>GPGSPITDERVYESIGQYGGETVKIVRIEKARDIPLGATVRNEMDSVIISRIVKGGAAEKSGLLHEGDEVLEINGIEIRGKDVNEVFDLLSDMHGTLTFVLIPSQQIKPPPAKETVIHVKAHFDYDPSDDPYVPCRELGLSFQKGDILHVISQEDPNWWQAYREGDEDNQPLAGLVPGKEEILTYEEMSLYHQPANRKRPIILIGPQNCGQNELRQRLMNKEKDRFASAVPHTTRSRRDQEVAGRDYHFVSRQAFEADIAAGKFIEHGEFEKNLYGTSIDSVRQVINSGKICLLSLRTQSLKTLRNSDLKPYIIFIAPPSQERLRALLAKEGKNPKPEELREIIEK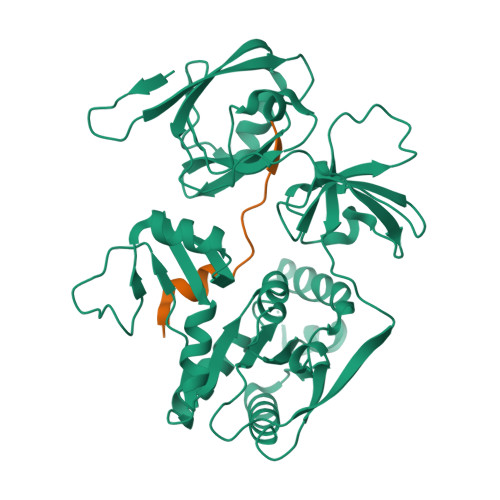TREMEQNNGHYFDTAIVNSDLDKAYQELLRLINKLDTEPQWVPSTWLR[2x];>[2x]GPGSEFRNKRATRGTYSPSAQEYCNPRLEMDNVLKPPPEERLI> VSKRAVITGLGIVSSIGNNQQEVLASLREGRSGIT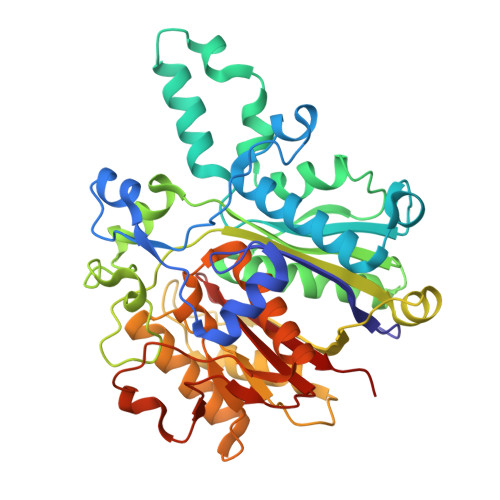FSQELKDSGMRSHVWGNVKLDTTGLIDRKVVRFMSDASIYAFLSMEQAIADAGLSPEAYQNNPRVGLIAGSGGGSPRFQVFGADAMRGPRGLKAVGPYVVTKAMASGVSACLATPFKIHGVNYSISSACATSAHCIGNAVEQIQLGKQDIVFAGGGEELCWEMACEFDAMGALSTKYNDTPEKASRTYDAHRDGFVIAGGGGMVVVEELEHALARGAHIYAEIVGYGATSDGADMVAPSGEGAVRCMKMAMHGVDTPIDYLNSHGTSTPVGDVKELAAIREVFGDKSPAISATKAMTGHSLGAAGVQEAIYSLLMLEHGFIAPSINIEELDEQAAGLNIVTETTDRELTTVMSNSFGFGGTNATLVMRKLK Here, we identify TECPR1 (tectonin beta‐propeller repeat containing 1) as a receptor for cytosolically exposed sphingomyelin, which recruits ATG5 into an E3 ligase complex that mediates lipid conjugation of LC3 independently of ATG16L1. TECPR1 is comprised of a central ATG5‐interacting region (AIR) and an adjacent pleckstrin homology (PH) domain with affinity for PI(3)P and/or PI(4)P (Chen et al, 2012; Wetzel et al, 2020). These domains are flanked by two 5‐bladed beta‐propellor domains, whose blades are formed from WD40‐like TECPR repeats. Inserted between the first and second blades of each propellor lie DysF domains, named after their occurrence in the protein Dysferlin and so far without known functions.

However, upon reductive methylation of primary amino groups, confirmed by matrix‐assisted laser desorption/ionisation (MALDI) time‐of‐flight (TOF) and in‐source decay (ISD) mass spectrometry (Fig EV3A and B), the N‐terminal DysF domain of TECPR1 yielded diffracting crystals, the structure of which was solved to 1.9 Å resolution by molecular replacement with the NMR structure of the inner DysF domain of myoferlin. The N‐terminal DysF domain of TECPR1 represents an elongated finger‐shaped domain, which, overall, bore high similarity to the inner DysF domains of myoferlin and dysferlin (Fig EV3C) (Patel et al, 2008; Sula et al, 2014a). The N‐terminal DysF domain of TECPR1 is comprised of a central pair of antiparallel beta strands connected via a long loop that wraps around the beta‐sheet and covers large parts of the domain surface. The loop is precisely positioned and held in place through planar stacking interactions between multiple tryptophan and arginine residues (specifically Trp 116, 118, 122, 138 and Arg 159, 161, 165, 167), a feature also found in Ferlin DysF domains (Patel et al, 2008; Sula et al, 2014a). Mutations of W77, L88, L89, I142, K152, K153 and W154 into alanine all abrogated recruitment, while mutations of I65, M80, E134, K135, T147, T149, K150, Y169 had little or no effect. Subsequent mutations of nearby residues R76, S90 and D143 into alanine and C84 and C157 into serine also abolished recruitment. Together these mutants identify a binding site located at the distal end of the domain, that is, the tip of the DysF finger. Consistent with the zwitterionic nature of sphingomyelin, the binding site is characterised by positively (R76, K152, K153) and negatively charged (D143), as well as hydrophobic residues. Notably, W77 and W154 are solvent‐exposed and upon binding may become inserted into target membranes. A comparison of the sphingomyelin‐binding site in the N'DysF domain of TECPR1 to the equivalent region in the inner DysF domains of myoferlin and dysferlin reveals little conservation of loop structures and exposed side chains, thus explaining why the latter domains are not recruited to damaged membranes.

>GAASDVPIRRREEAYENQRWNPMGGFCEKLLLSDRWGWSDVSGLQHRPLDRVALPSPHWEWESDWYVDENFGGEPTEKGGWTYAIDFPATYTKDKKWNSCVRRRKWIRYRRYKSRD[3x]6-(2-{3-fluoro-5-[3-(methylamino)prop-1-yn-1-yl]phenyl}ethyl)-4-methylpyridin-2-amine 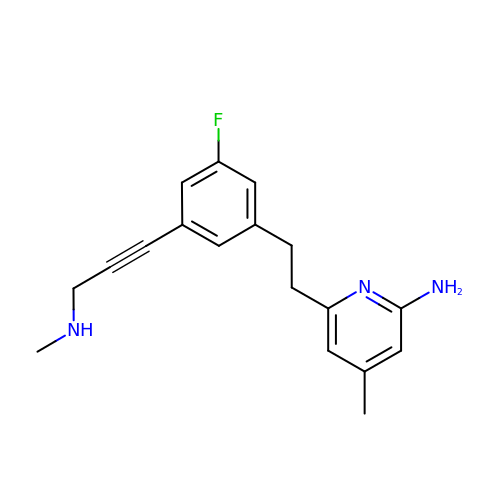| C18 H20 F N3 | YNFSNSWWKPMRND-UHFFFAOYSA-N>HHHHHHSSGLVPRGSHMAISHVQLFSVPVSDQEKAKDFYVETVGFDLLADQPGVHGRWLQVAPKGADTSLVLVDWFPTMPPGSLRGLLLRTDDVDADCARLQERGVAVDGPKNTPWGRQAMFSDPDGNVIGLNQPSASAG[2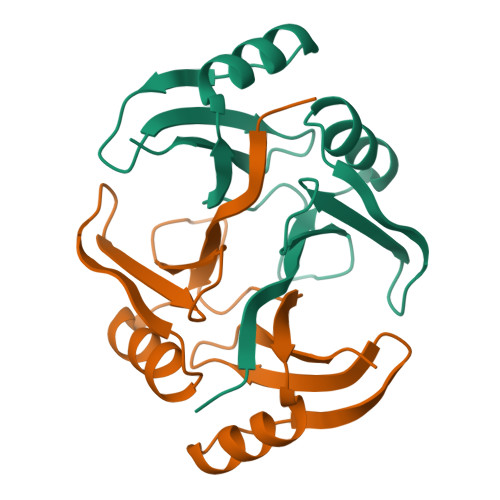x]> MLKRLQVKNFRCLEDIDLPLGPLTAIVGPNGAGKTTILRAIDLVLGDVWPSLRSFRIPQDFINFDTTRAIEITVHFDPPYTQGSFNITAFRLTCKGEDADFHVDLEPLDEGGNVPRYPSGNPLRVGTDMRNHARVLFLDHRRNLAQHLPSIRGSILGRLLQPVRREFKLQDNFKQVYEQAMDLLRTEQVKQIEKTIAETAKQMLGFLGKDAMKSMEIGFGFADPANPFNSLRLQYRESDLTLPGDELGLGIQSAIVVGIFEAFRQLGEKIGTVIIEEPEMYLHPQAQRYFYRLLCEMADKDQCQIIYSTHSPIFADVNRFEALRLVRKDRDDRVVVSYVREEDKSALDNVRNRFKLGGRFDTARNEVLFAKRALLVEGYGDRVAALQLFNQLEVDPDAECIAVVDCGGKAGIELIVGVCKALDIPFVVVHDEDVWPIDERADEETRRKQEQENKAEQEKNQRIQACAGAERVFVVQPSLEAALGIGRNASDKPYRIAEILKTVDVGQPPDALRPFVEAIRQVTRPMEE

Overcoming lysogenization defect (OLD) proteins comprise a poorly characterized family of nucleases that contain an N-terminal ATPase domain and C-terminal Topisomerase/Primase (Toprim) catalytic domain. OLD homologs are widely conserved in bacteria, archaea and some viruses and can be subdivided into two classes. Class 1 OLD homologs exist as single, isolated genes while Class 2 old genes always appear in tandem with a UvrD/PcrA/Rep-like helicase. Here, we present the crystal structure of a full-length Class 1 OLD nuclease from Thermus scotoductus (Ts) at 2.20 Å resolution.

Optimized crystals of native TsFL routinely diffracted beyond 2.5 Å and structure was solved by SAD phasing using a platinum soaked derivative. The resulting model was refined to 2.20 Å and contained residues 1–142, 149–237 and 245–525. TsFL subunits are comprised of three structural domains: an N-terminal ATPase domain, a helical dimerization domain, and a C-terminal Toprim domain. The dimerization domain inserts between the β8 and β9 strands of the ATPase domain and consists of four helices (α1D, α2D, α3D and α4D) that form a kinked structure. α1D, α2D and α4D from each subunit directly associate in trans at the dimer interface while α3D bends back and rests on top of α4A and α5A. Together these interactions form an extensive hydrophobic network that buries 3479 Å2 of surface area and maintains the tight association between the subunits. The amphipathic α2T helix packs against a hydrophobic groove on the edge of ATPase domain formed by α6A, α7A, α8A and β11A to bury 920Å2. Despite attempts to co-crystallize with ATP analogs, only a sulfate ion deriving from the crystallization buffer was present in the TsFL active site. The sulfate binds in the position normally occupied by the β-phosphate of ATP and forms stabilizing hydrogen bonds with the main chain atoms of G31, G33 and K34 and the side chain hydroxyl of T35. Ts residues E377, D431 and D433 align with the Bp OLD metal A binding residues E400, D455, and D457 while D381, S478, E480 roughly superimpose with the Bp metal B ligands E404, T506 and E508. These residues are conserved among all Class 1 homologs and in the TsFL structure coordinate a single samarium ion from the crystallization conditions. The trans-acting catalytic side chain H283 of the Ts OLD D loop is far removed from the composite active site in this arrangement—displaced nearly 46 Å (Cα to Cα) from the respective position of its counterpart (D953) in Mj Rad50 —and would be unable to exert its functional effects efficiently. This suggests that the TsFL conformation captured in the crystal is non-productive for ATPase hydrolysis and would require additional conformational rearrangements, likely triggered by nucleotide binding, to achieve a more canonical organization of the ATPase domains.>[4x]MGSDKIHHHHHHENLYFQGMNF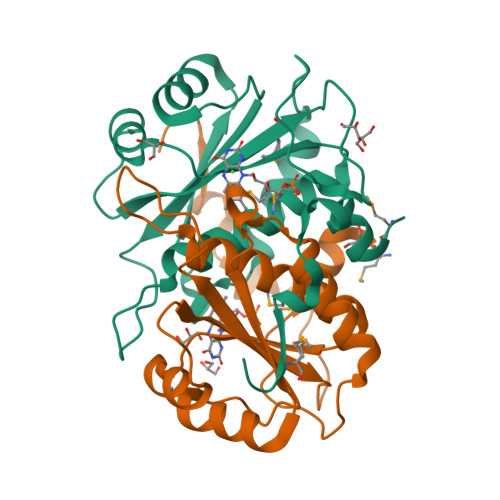VELAKKRYSCRNYQDRKVEKEKLEKVLDVARIAPTGGNRQPQRLIVIQEKEGINKLSKAANIYDAPLAILVCGDKDKVWTRPFDGKQLTDIDTSIVTDHMMLQATELGLASVWVCYFNPDIIREEFSLPDNLEPINILLMGYESKIPESPERHEKTRVPLSEIVSYETL> MKPLVHVASVEKGRSYEDFQKVY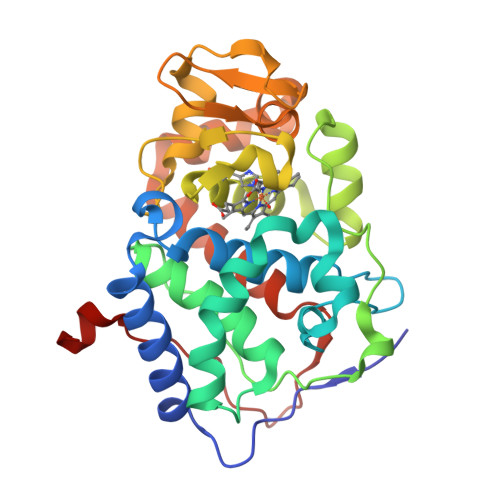NAIALKLREDDEYDNYIGYGPVLVRLAWHTSGTWDKHDNTGGSYGGTYRFKKEFNDPSNAGLQNGFKFLEPIHKEFPWISSGDLFSLGGVTAVQEMQGPKIPWRCGRVDTPEDTTPDNGRLPDADKDADYVRTFFQRLNMNDREVVALMGAHALGKTHLKNSGYEGPWGAANNVFTNEFYLNLLNEDWKLEKNDANNEQWDSKSGYMMLPTDYSLIQDPKYLSIVKEYANDQDKFFKDFSKAFEKLLENGITFPKDAPSPFIFKTLEEQGL>NKICQFKLVLLGESAVGKSSLVLRFVKGQFHEFQESTIGAAFLTQTVCLDDTTVKFEIWDTAGLERYHSLAPMYYRGAQAAIVVYDITNEESFARAKNWVKELQRQASPNIVIALSGNKADLANKRAVDFQEAQSYADDNSLLFMETSAKTSMNVNEIFMAIAKKLPK[2x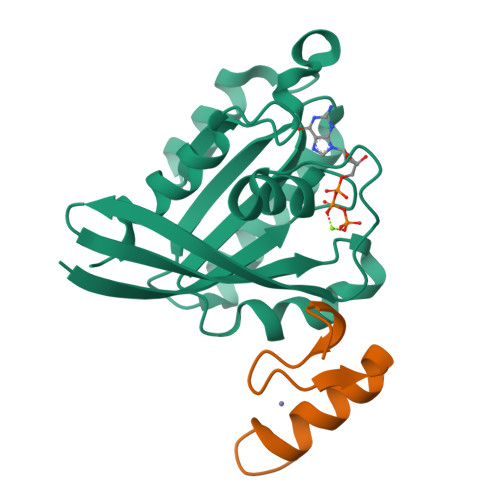];>[2x]SSSEGFICPQCMKSLGSADELFKHYEAVHDAGND> MQKHNEDLKESFLLFDGDGDGYLTLNEFESLVRVLG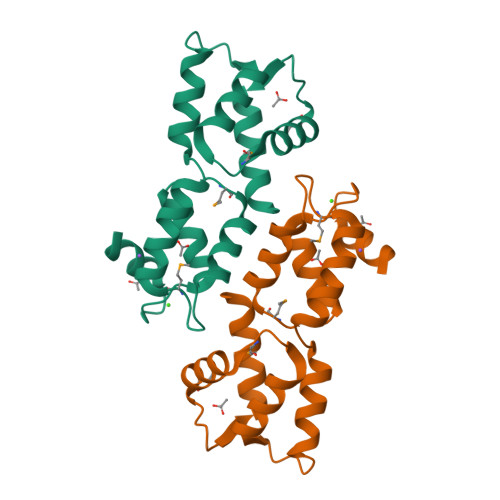VVMETSAIASTYNSNSKVRGMSYELFTSCFSQLKTKSFNKDEIKTAINVLDKDKKGFIPAIELRRILSTIGDNMEQKEITDLFTFMGIDEQGVVKVDDFINQDNHHHHHH>MRGSHHHHHHTDPIMKPENKLPVLDLISAEMKTVVNTLQPDLPPWPATGTIAEQRQYYTLERRFWNAGAPEMATRAYMVPTKYGQVE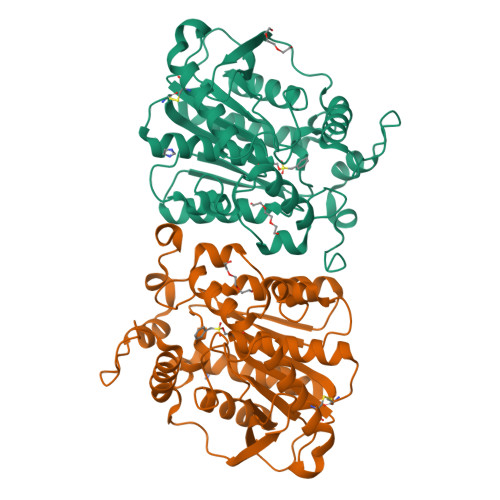TRLFCPQPDSPATLFYLHGGGFILGNLDTHDRIMRLLASYSQCTVIGIDYTLSPEARFPQAIEEIVAACCYFHQQAEDYQINMSRIGFAGDSAGAMLALASALWLRDKQIDCGKVAGVLLWYGLYGLRDSVTRRLLGGVWDGLTQQDLQMYEEAYLSNDADRESPYYCLFNNDLTREVPPCFIAGAEFDPLLDDSRLLYQTLAAHQQPCEFKLYPGTLHAFLHYSRMMKTADEALRDGAQFFTAQL[6x]> MNWLFLVSLVFFCGVSTHPALAMSSNRLLKLANKSPKKIIPLKDSSFENILAPPHENAYIVALF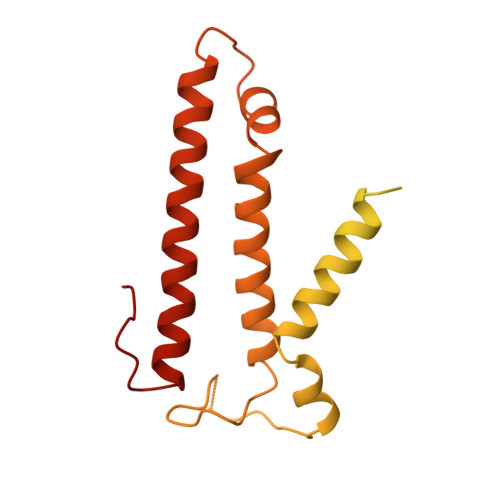TATAPEIGCSLCLELESEYDTIVASWFDDHPDAKSSNSDTSIFFTKVNLEDPSKTIPKAFQFFQLNNVPRLFIFKPNSPSILDHSVISISTDTGSERMKQIIQAIKQFSQVNDFSLHLPMDWTPIITSTIITFITVLLFKKQSKLMFSIISSRIIWATLSTFFIICMISAYMFNQIRNTQLAGVGPKGEVMYFLPNEFQHQFAIETQVMVLIYGTLAALVVVLVKGIQFLRSHLYPETKKAYFIDAILASFCALFIYVFFAALTTVFTIKSPAYPFPLLRLSAPFK>SNAMKFEAVVRTELGKGASRRLRLAGQFPAVVYGGEAAPVAVALNHDDIVNQMDKPEFYEAITLVIGGEEVKVKP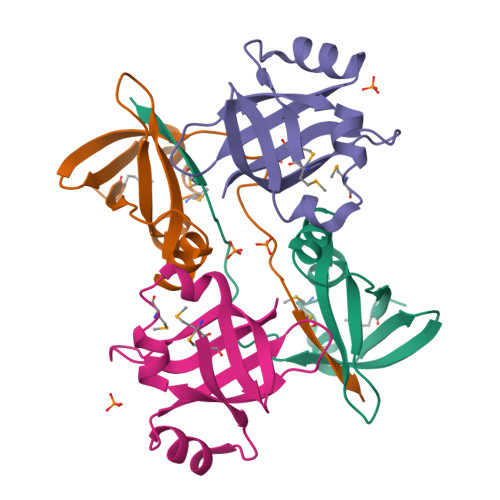QDVQRHAFKPKVEHMDFIRI[8x]> MSKKSDAIKQTKSFSILLMGVDTGSSERTSQWEGNSDSMILVTVNPETKKTTMTSLER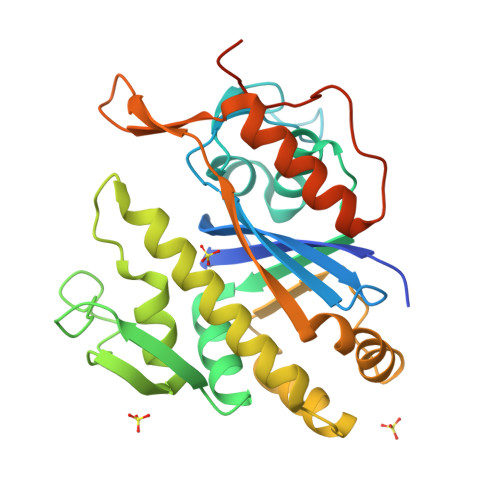DILITLSGPKNNDMNGAEAKLNAAYAAGGAQMAIMTVQDLLNITIDNYVQINMQGLIDLVDAVGGITVTNEFDFPISIADNEPEYQATVAPGTHKVNGEQALVYARMRYDDPEGDYGRQKRQREVIQKVLKKILALDSISSYRKILSAVSGNMQTNIEISSNTIPGLLGYRDALKTIKTYQLKGEDATLSDGGSYQIVTSDHLLETQNRIRGELGLRKVTQLKTSATVYENLYGSRKSALEHHHHHH Endo-β-N-acetylgucosaminidases (EC 3.2.1.96) (ENGases) are a class of enzymes that hydrolyze the glycosidic bond - GlcNAc β-1,4GlcNAc - present in N-linked sugar chains in glycoproteins and release the N-glycan moiety. Endo-A from Arthrobacter protophormiae is modular in architecture with three distinct domains. Domain 1, with residues 2–350 being identified, is the largest and displays a typical (β/α)8 TIM barrel fold, which has been observed for proteins belonging to family GH18 and GH20 of the glycoside hydrolases. Endo-A catalyses hydrolysis and transglycosylation via a substrate-assisted mechanism, in which the C2 acetamido group mounts a nucleophilic attack at the anomeric carbon resulting in the formation of an oxazoline ion intermediate.

In summary, we have determined the crystal structure of Endo-A, the first representative structure for members of the GH85 family of hydrolases. The overall architecture of the domain 1 is similar to that observed in the structure of Endo-F3. In addition, the structure of Endo-A reveals two smaller domains, primarily made up of β sheets. The secondary structural elements of these two domains are interdigitated. In the structure of ligand-free Endo-A, H2O846 is interacting with Y205 and could fulfill the role of a potential nucleophile. Analysis of the structure of Endo-A reveals that the Y205F mutation probably results in loss of a potential nucleophile, H2O846, which is hydrogen bonded to the hydroxyl oxygen of Y205. In the structures of the free Endo-A and Endo-A bound to Man3GlcNAc-thiazoline, the side chain of W244 is perpendicular to W216 and introduces a steric block at the entrance of the active site. The overall structures of the Endo-A in complex with Man3GlcNAc-thiazoline and Endo-A in complex with GlcNAc-Asn are identical to that of the free protein.

>STYNGPLSSHWFPEELAQWEPDSDPDAPFNRSHVPLEPGRVANRVNANADKDAHLVSLSALNRHTSGVPSQGAPVFYENTFSYWHYTDLMVYWAGSAGEGIIVPPSADVIDASHRNGVPILGNVFFPPTVYGGQLEWLEQMLEQEEDGSFPLADKLLEVADYYGFDGWFINQETEGADEGTAEAMQAFLVYLQEQKPEGMHIMWYDSMIDTGAIAWQNHLTDRNKMYLQNGSTRVADSMFLNFWWRDQRQSNELAQALGRSPYDLYAGVDVEARGTSTPVQWEGLFPEGEKAHTSLGLYRPDWAFQSSETMEAFYEKELQFWVGSTGNPAETDGQSNWPGMAHWFPAKSTATSVPFVTHFNTGSGAQFSAEGKTVSEQEWNNRSLQDVLPTWRWIQHGGDLEATFSWEEAFEGGSSLQWHGSLAEGEHAQIELYQTELPISEGTSLTWTFKSEHDNDLNVGFRLDGEEDFRYVEGEQRESINGWTQWTLPLDAFAGQTITGLAFAAEGNETGLAEFYTGQLAVGADSEKPAAPNVNVRQYDPDPSGIQLVWEKQSNVHHYRVYKETKHGKELIGTSAGDRIYIEGLVEESKQNDVRLHIEALSETFVPSDARMIDIKSGSF[4x]> GSD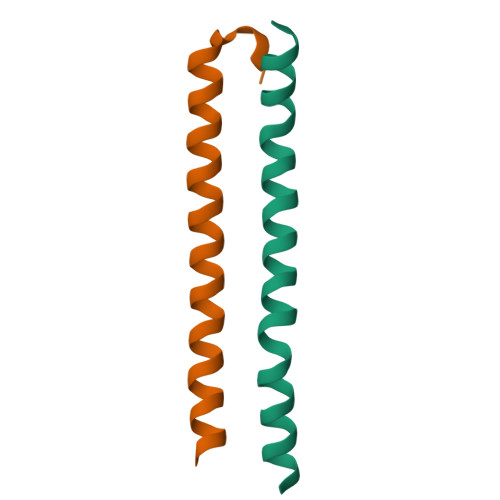YEFLKSWTVEDLQKRLLALDPMMEQEIEEIRQKYQSKRQPILDAIEAK;> GSEVEWDAFSIPELQNFLTILEKEEQDKIQQVQKKYDKFRQKLEEALRESQGKPG> MSHHHHHHSMDIELMKIDILDKGFVELVDVMGNDLSAVRAARVSFDMGLKDEERDRHLIEYLMKHGHETPFEHIVFTFHVKAPIFVARQWFRHRIASYNELSGRYSKLSYEFYIPSPERLEGYKTTIPPERVTEKISEIVDKAYRTYLELIESGVPREVARIVLPLNLYTRFFWTVNARSLMNFLNLRADSHAQWEIQQYALAIARIFKEKCPWTFEAFLKY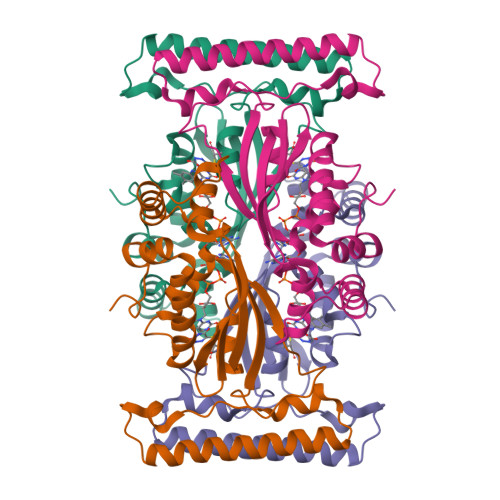AYKGDILKEVQV(3R)-6,8-dihydroxy-3-{[(2R,6R)-6-methyloxan-2-yl]methyl}-3,4-dihydro-1H-2-benzopyran-1-one | C16 H20 O5 | 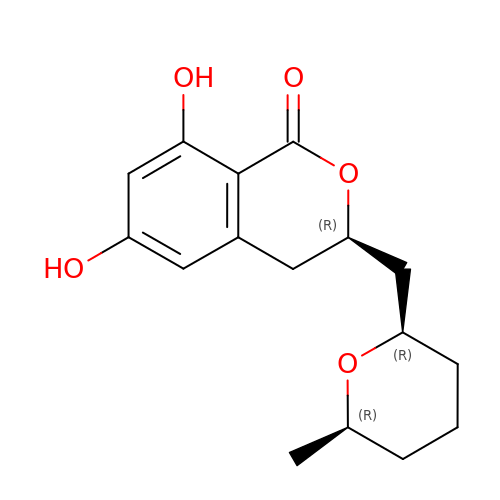WOMKDMUZNBFXKG-OASPWFOLSA-N> TKNPKLFISSTWMSHMTMPTENTDGEESLTSSKQQQQQSGDKHMEPLGTDDDFWGPSGPVSTEVVDRERNLYRVRLPMAGSYHCPSTGLHFV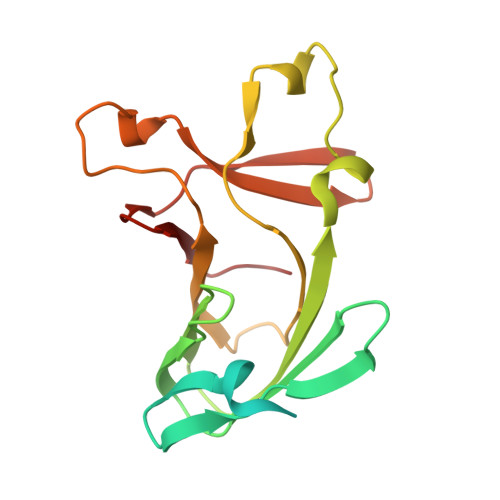VTRAVTIEIGFCAWSQFLHETPLQHSHMVAGPLFDIKAEHGAVTAVCLPHFVSLQEGKVDSSLFHVAHFQDHGMVLETPARVEPHFAVLENPSF> QFMNKQRTLLISSRGVNYRHRHLIQDLSGLLPHSRKEPKLDTKKDLQQLNEIAELYNCNN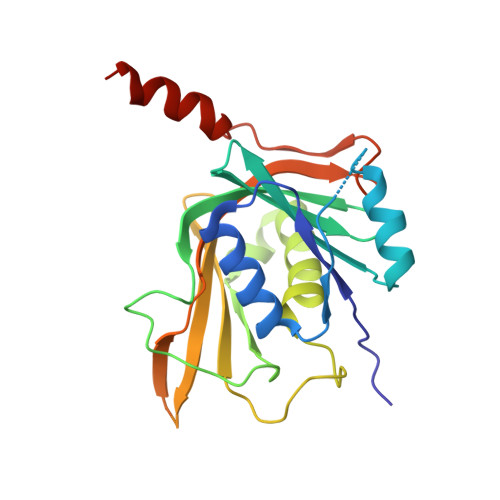VLFFEARKHQDLYLWLSKPPNGPTIKFYIQNLHTMDELNFTGNCLKGSRPVLSFDQRFESSPHYQLIKELLVHNFGVPPNARKSKPFIDHVMSFSIVDDKIWVRTYEISHSTKNKEEYEDGEEDISLVEIGPRFVMTVILILEGSFGGPKIYENKQYVSPNVVRAQIKQQAAEE> MSLENKFARTVLGDIPVEKLGITDCHDHFIKNGGPEVEEHIDFLMLNVDASIKEFKEFIDRGGSTIVTMDPPNVGRDVLKTLEIANAVKNLGGNVIMSTGFHKAKFYDKYSSWLAVVPTEEIVKMCVAEIEEGMDEYNYNGPVVKRSKAKAGIIKAGTGYGAIDRLELKALEVAARTSILTGCPILVHTQLGTMALEVAKHLIGFGANPDKIQISHLNKNPDKYYYEKVIKETGVTLCFDGPDRVKYYPDSLLAENIKYLVDKGLQKHITLSLDAGRILYQRNYGLTKGKQTFGLAYLFDRFLPLLKQVGVSKEAIFDILVNNPKRVLAFDEKRNFDPLKVSKEV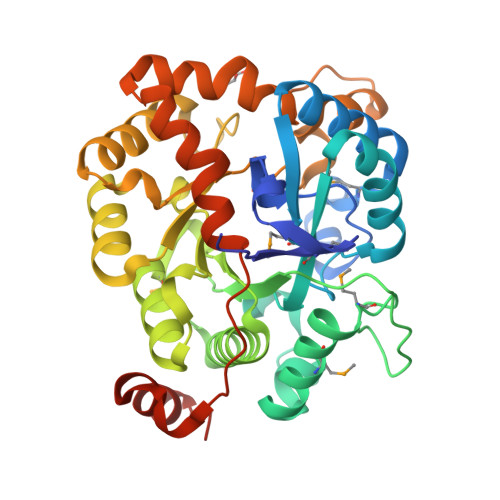LELKKELNLNEGHHHHHH>[2x]GMGKRILLLEKERNLAHFLSLELQKEQYRVDLVEEGQKALSMALQTDYDLILLNVNLGDMMAQDFAEKLSRTKPASVIMILDHWEDLQEELEVVQRFAVSYIYKPVLIENLVARISAIFRGRDFIDQHCSLMKVPRTYRNLRIDVEHHTVYRGEEMIALTRREYDLLATLMGSKKVLTREQLLESVWKYESATETNIVDVYIRYLRSKLDVKGQKSYIKTVRGVGYTMQEG

Here we describe the two-component-like orphan response regulator RitR (Repressor of iron transport Regulator) as the archetype of a novel family of peroxide-sensing transcription factors in the pneumococcus and related species. RitR contains an Aspartate-less Receiver (ALR) REC-like domain, which retains the common (α/β) fold of canonical REC versions, yet lacks “invariant” residues in its catalytic pocket required for typical phosphotransfer, including the phospho-accepting Asp residue crucial for the histidine kinase-response regulator phosphorelay.. Here we show that RitR regulates pneumococcal iron homeostasis in response to cellular peroxide concentrations through its single Cys (Cys128) located within the linker domain of the protein. Atomic structures of RitR in its oxidized and reduced states demonstrate a dramatic mechanism of activation that hinges on the helical unraveling and subsequent formation of an inter-protomer disulfide bridge to enable DNA binding and transcriptional regulation of Piu.

To observe structural rearrangements after RitR oxidation at the atomic level, we purified, crystallized and solved the atomic structure of native wild-type RitR in the peroxide-induced oxidized, free dimeric form. Because the individual protomers of RitROX were sufficiently close to the RitRC128S structure, the dimeric RitROX structure could be largely solved using molecular replacement (structural statistics can be found in Table 1). At least in the absence of its DNA target sequence, the oxidized RitR structure revealed that its individual domains do not change significantly upon oxidation with H2O2. However, the relationship between protomers changes dramatically, whereupon oxidation, as predicted, the DNA-binding domain is released from the α4-β5-α5 interface of the REC domain. In the absence of its interacting DNA, the final result of the free form of oxidized RitR produces an unusual domain-swapped structure, i.e. where the DNA binding domain from protomer 1 binds to the RD of protomer 2 and vice versa. Importantly, the RitROX swapped domain structure is possible due to the effective unwinding of the C-terminus of the linker (α5 helix) to free Cys128, enabling it to form the inter-protomer disulfide bridge, and unequivocally showing that Cys128 is responsible for dimer formation. Aside from the Cys128-Cys128' linkage and the adjacent Ser129 forming a main chain nitrogen bond to the hydroxyl side chain of Ser129' in the other protomer, there are few observable electrostatic interactions between swapped dimers to hold the conformer together. However, a comparison of average B-factors between the RitRC128S and RitROX structures revealed that although REC-DBD interactions appear almost identical in their 3-dimensional atomic coordinates, there are major differences in their average residue B-factor values, where the RitRC128S and RitROX structures exhibit average alpha carbon B-factors of 11.03 and 36.25, respectively.>MNTPEHMTAV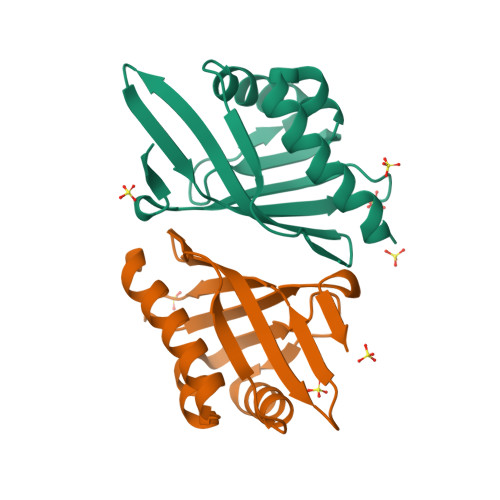VQRYVAALNAGDLDGIVALFADDATVEDPVGSEPRSGTAAIREGYANSLKLPLAVELTQEVRAVANEAAFAFTVSFEYQGRKTVVAPIDHFRFNGAGKVVSMRALFGEKNIHAGA[4x]>[2x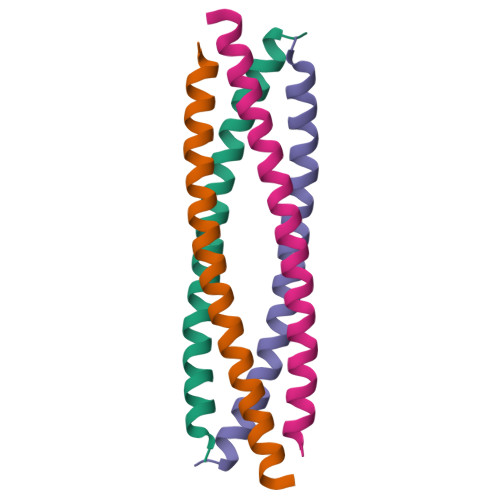]EFSQLLALASLLGQQQAEVQRCREDLQKKESLVMETIAKIKALALEHHHHHH N',N''-{furan-2,5-diylbis[3-(piperidin-4-yloxy)benzene-4,1-diyl]}dipyridine-2-carboximidamide | C38 H40 N8 O3 | 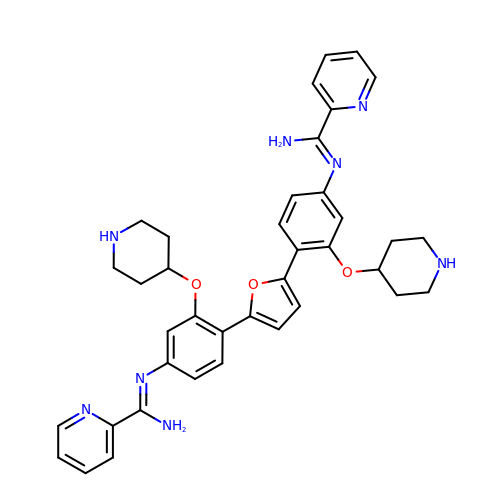ZOPMAKJQIUYLIW-UHFFFAOYSA-N(2-cyclohexyl-1,3-benzoxazol-6-yl){3-[4-(pyrimidin-2-yl)piperazin-1-yl]azetidin-1-yl}methanone | C25 H30 N6 O2 | 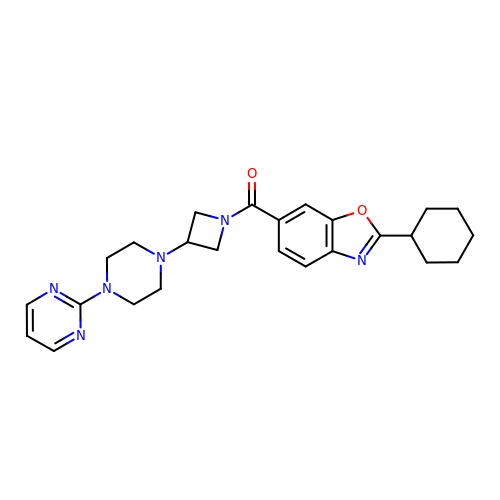IABLYMUVWHQTGC-UHFFFAOYSA-N> AVGPVTDIHIVNKDIAPDGFSRPSVLAGGTFPGPLITGQKGDNFKLNVVDDLTDA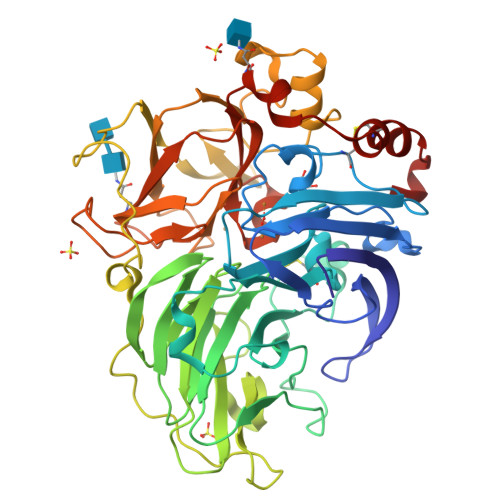SMLKSTSIHWHGFFQKGTNWADGPAFVNQCPISTGNSFLYNFQVPDQAGTYWYHSHLSTQYCDGLRGAFVVYDPTDPHKALYDVDDESTVITLADWYHTLARQIVGVAIADTTLINGLGRNTNGPADAALAVINVEAGKRYRLRLVSISCDPNYVFSIDNHDFNIIEVDGVNSKPLNVDSIQIFAGQRYSAVLNANQPVGNYWVRANPNLGTTGFTGGINSAILRYKGAPVAEPTTTQTTSTKPLQEPNLRPLVSMPVPGSATPGGVDVVHNLILGFSAGKFTINGAAFTPPSVPVLLQILSGTTNAQDLLPSGSVITLPIGKTIELTLAAGVLGGPHPFHLHGHNFHVVRSAGQTTPNYVDPIVRDVVNTGGTGDNVTIRFTTDNPGPWFLHCHIDWHLEAGFAVVFAEGVNQTNAANPTPADWNNLCNIYNALADGDK>MSNDHPQPLDAAEIPRFAGIPTFMRLPAFTDPAALQVGLIGVPWDGGTTNRAGARHGPREVRNLSSLMRKVHHVSRIAPYDLVRVGDLGDAPV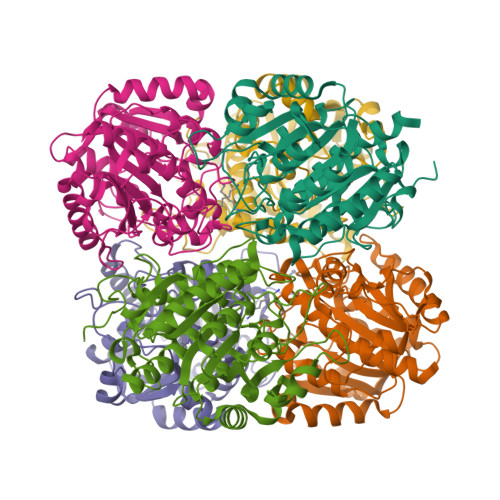NPIDLLDSLRRIEGFYRQVHAAGTLPLSVGGDHLVTLPIFRALGRERPLGMVHFDAHSDTNDRYFGDNPYTHGTPFRRAIEEGLLDPLRTVQIGIRGSVYSPDDDAFARECGIRVIHMEEFVELGVEATLAEARRVVGAGPTYVSFDVDVLDPAFAPGTGTPEIGGMTSLQAQQLVRGLRGLDLVGADVVEVSPPFDVGGATALVGATMMFELLCLLAESAARSALEHHHHHH[6x]> MAEKEEAIFRSAEMALVQFYIPQEISRDSAYTLGQLGLVQFRDLNSKVRAFQRTFVNEIRRLDNVERQYRYFYSLLKKHDIKLYEGDTDKYLDGSGELYVPPSGSVIDDYVRNASYLEERLIQMEDATDQIEVQKNDLEQYRFILQSGDEFFLKGDNTDSTSYMDEDMIDANGENIAAAIGASVNYVTGVIARDKVATLEQILWRVLRGNLFFKTVEIEQPVYDVKTREYKHKNAFIVFSHGDLIIKRIRKIAESLDANLYDVDSSNEGRSQQLAKVNKNLSD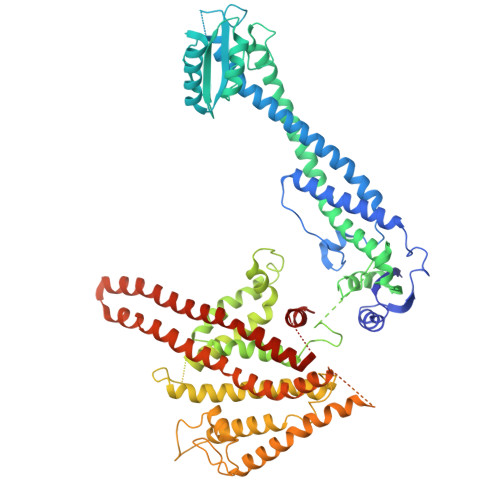LYTVLKTTSTTLESELYAIAKELDSWFQDVTREKAIFEILNKSNYDTNRKILIAEGWIPRDELATLQARLGEMIARLGIDVPSIIQVLDTNHTPPTFHRTNKFTAGFQSICDCYGIAQYREINAGLPTIVTFPFMFAIMFGDMGHGFLMTLAALSLVLNEKKINKMKRGEIFDMAFTGRYIILLMGVFSMYTGFLYNDIFSKTMTIFKSGWKWPDHWKKGESITATSVGTYPIGLDWAWHGTENALLFSNSYKMKLSILMGFIHMTYSYFFSLANHLYFNSMIDIIGNFIPGLLFMQGIFGYLSVCIVYKWAVDWVKDGKPAPGLLNMLINMFLSPGTIDDELYPHQAKVQVFLLLMALVCIPWLLLVKPLHFKFTHKKKSHEPLPSTEADASSEDLEAQQLISAMDADDAEEEEVGSGSHGEDFGDIMIHQVIHTIEFCLNCVSHTASYLRLWALSLAHAQLSSVLWTMTIQIAFGFRGFVGVFMTVALFAMWFALTCAVLVLMEGTSAMLHSLRLHWVESMSKFFVGEGLPYEPFAFEYKDMEVAVASASSSASS Pannexins are a family of ubiquitously expressed large-pore forming channels which regulate nucleotide release during apoptosis, blood pressure, and neuropathic pain. Among the pannexin family, pannexin 1 (Panx1) has garnered the most attention for its role as a large-pore forming channel responsible for ATP release from a variety of cell types. Different kinds of stimuli have been reported to activate Panx1 including voltage, membrane stretch, increased intracellular calcium levels, and positive membrane potentials. Like other large-pore forming channels, each Panx1 protomer harbors four transmembrane helices (TM1-4), two extracellular loops (ECL1 and 2), two intracellular loops (ICL1 and 2), and an amino (N)-terminal loop.

We further stabilized frPanx1 by truncating the C-terminus by 71 amino acids and by removing 24 amino acids from the intracellular loop between transmembrane helices 2 and 3. Purified frPanx1-ΔLC was reconstituted into nanodiscs composed of MSP2N2 (an engineered derivative of apolipoprotein) and soybean polar lipids, and subjected to cryo-electron microscopy (cryo-EM) and single-particle analysis. We used a total of 90,185 selected particles for 3D reconstruction at 3.0 Å resolution. The map quality was sufficient for de novo model building for the majority of frPanx1-ΔLC with the exception of disordered segments of the N-terminus (residues 1–10), ECL1 (88–100), and ICL1 (157–194). The frPanx1-ΔLC structure revealed a heptameric assembly, which is unique among the known eukaryotic channels. The Panx1 permeation pathway spans a length of 104 Å, with constrictions formed by the N-terminal loop, Ile58, and Trp74. The narrowest constriction is surrounded by Trp74 located on ECL1. We observed that the distance between the guanidino group of Arg75 and the benzene ring of Trp74 from an adjacent subunit is ~4 Å, suggesting that these two residues likely participate in an inter-subunit cation-π interaction key to Panx1 ion selectivity. Mapping such residues in the Panx1 structure revealed that they are clustered proximal to the extracellular constriction by Trp74, in a groove formed between ECL1 and ECL2. Based on the lack of channel activity at 0 mV, our current structure may represent a closed conformation.

>[7x]MAIAHIATEYVFSDFLLKDPPESKYKGLRLELAVDKLVSCIAVGLPLLLISLAFAQEITLGSQISCFAPTSFSWRQAAYVDSFCWAAVQQKHLSQSDSGNVPLWLHKFFPYILLLVAVLLYLPNLFWRFTAAPHLSSDLKFVMEELDKCYNRDIKDIKAANNLNSSDKRDYPIVEQYLKTKNNSYGLIIKYLICRVVTLIIVFTACIYLGYYISLFSLTDEFTCNIRTGILRNDTALPPLVQCKLIAVGVFRLLSYINLIIYVLIMPFIIYAMLVPFRKTANVLKVYEVLPTFSVQQAPSKTYDDHSLFLLFLEENVSELKSYKFLKVLENIKASSWSHPQFEK> GSHMAKPLTDSEKRKQISVRGLAGLGDVAEVRKSFNRHLHFTLVKDRNVATPRDYFFALAHTVRDHLVGRWIRTQQHYYERDPKRIYYLSLEFYMGRTLQNTMVNLGLQNACDEAIYQLGLDLEELEEIEEDAGLGNGGLGRLAACFLDSMATLGLAAYGYGIRYEFGIFNQKIVNGWQVEEADDWLRYGNPWEKARPEYMLPVHFYGRVEHTPDGVKWLDTQVVLAMPYDTPVPGYKNNTVNTMRLWSAKAPNDFKLQDFNVGDYIEAVLDRNLAENISRVLYPNDNFFEGKELRLKQEYFVVAATLQDIIRRFKSSKFGCRDPVRTCFETFPDKVAIQLNDTHPALSIPELMRILVDVEKVDWDKAWEITKKTCAYTNHTVLPEALERWPVSMFEKLLPRHLEIIYAINQRHLDHVAALFPGDVDRLRRMSVIEEGDCKRINMAHLCVIGSHAVNGVARIHSEIVKQSVFKDFYELEPEKFQNKTNGITPRRWLLLCNPGLADTIVEKIGEEFLTDLSQLKKLLPLVSDEVFIRDVAKV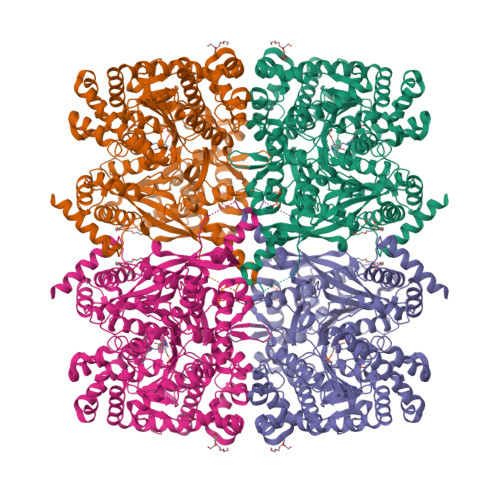KQENKLKFSAFLEKEYKVKINPSSMFDVHVKRIHEYKRQLLNCLHVVTLYNRIKRDPAKAFVPRTVMIGGKAAPGYHMAKLIIKLVTSIGDVVNHDPVVGDRLKVIFLENYRVSLAEKVIPAADLSQQISTAGTEASGTGNMKFMLNGALTIGTMDGANVEMAEEAGAENLFIFGLRVEDVEALDRKGYNAREYYDHLPELKQAVDQISSGFFSPKEPDCFKDIVNMLMHHDRFKVFADYEAYMQCQAQVDQLYRNPKEWTKKVIRNIACSGKFSSDRTITEYAREIWGVEPSDLQIPPPNIPRD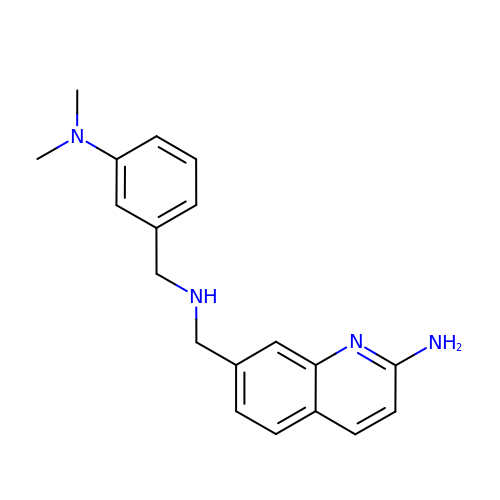7-[[[3-(dimethylamino)phenyl]methylamino]methyl]quinolin-2-amine | C19 H22 N4 | SOVIURHDFSQRNW-UHFFFAOYSA-N> MVTVTDPLTARLEAAIKAWSDFFSDAEHERLDPAIFADQSQTLFANHPLAPVPLADLLLRPTPSNRECVDQRTLQYLQVLQKQGRITTAAVLRALYKYSTAHTRAQTPDGKPKHGAGDSSTNDADVGGSSKADLTSRMVRWRNSYMVEEDVLWRLARAVNHGTGIKTSHDVTEVAKVLARWTALFAEVSAAISRDAFNSMNGLQVKDESEDARNAFVLFYFAFCENQIVNETLSQPVCKDICRKLLDSLDAFLPTLMHLTADITGRLEHFRSEVLARYAPQEKKSMDMPSFMNDLSMSLESFQVPELPVVNTRAGLYIYLGAALVGRPMIDDEALFSYLHNRYQGDLQAMAVHLILASFDLLANAVFRNEGAKTGHLLKSFLINKVPLILVQLVAYAATTMYPFNAEMCITEALNQVDINMFPTLSGMFDMPNNNSFNDSVRQDFCFACQLHGLLSQAAIETLLGDITYQSLPPEGRYVKEQLVQACLQEPDRTLKLIGELDNMNGNVGAAAQAIVEICRDLASKPLSLDVLLLFDKPHKILHPLCELLDNWAGYEEDHGEYQPVYEEFGSVLLLLLAFVYRYNLSTADLGIRSSGSFVAKLLNGVDRCQPLEQLSEQEKSHLGGWIHGLFDTEAGGLGDELMSSCPPQDFYLLAPTLFHQIVNALSAGYLTDEMLKGGLEYLVDVLLLPALVPALLYLSNLLWADNQPIQNAVIKILQPILKPTSISNEASTMLSSVLNIVAKPLEHALKSYQRQDPECQKIEPLLLAIADNLAVSRRTGGADHTELESWCSAQITNPATGALIHGGLAAAVRTTIQQLVQWAQNPTLNSMNGMPAPYTHRQTLAAQQILGPHRLLGIILDELKSSPEPGIAYDVVTTMICAPDVRNSTISSPSTQSNNSSDHNDQAQNHQSQDAKHKHPHRLTLRDALRLEAHDFRAHLRADPVLAETVVRLYRRVEAQLTPLALPLPPAAAAAPAVGVNVGVDAATAAAAAAAAAMMPDALGLGVVGGVELGGMEGAIAAAVAAANGSGTGGAGGDGTQGGAGDAGMGLDGQQQGQGGSSAGDMGLGGGTADDIFSGLSGPDDFGADFGSWSMDLS;> MEARAHGALPNNYDRERFINGVGGDDKALKRKLEEPLSDITKELDTVIAQSDVAVADPKGQLCPDADVPDEMEHITDGILPLNLLLIRLAEFSHSKLEELVTMLASKPVPQHAVNGNGSHSTLVEDASPESQEKKRLLLNTIQDLHSRWVKALVITEWARNAEKVGKLIDIRTHLFKKLELYPQVLNDFINLKRDMAWAKVPSPDLKTALHILTHGEVTWMPDFNFLDPPPLTTEETLRWINDMNLALHARLQLEEHDKLPPPFKNYTIDSGRVTFRVRGEFEVDLSISEEDFSEQFWFINFRFDFSPAPAELTPAVRYWMTEKVNNILKTEGLGGCYKYLHEFTLTQKIAELHRQAIALNKGRWANSLRVEKLNRNLGIHYWANRLHSQNLKSWIIIGVHSGEDPQGLEEPKPSYLMVQWFREGVEQFIDIPFSQEKLSIEEILEFVTAKHVGYLLFSLFRKFDGKPRFTQGKKARLELNVWTQKPEDYYLSMQLLDDEDLKIQVNPWMGDFITTPSTGPWNRTLNSLGNPAEEGSKELENFRYIYIISVLKAQGKSHGWSVVRSPISQDELRSIVHSESASSRETFQAAWTRFVDWDPQWYAMRSMSLAGDQWWLVEVTSQRQSISGNRLVFFTKMAPCFSEERLTDGFFNGLRDHSRRLIAEITNLRELYPGITPSQLRKLIDPTRQPPVLPVKASKILGDFGGADAQSIAWLKDPVWLIYRGSACDTRVSDSPQQKRTQPVLDVFEAYLDVTDRRRFQTLNPRLDRDILYNPYTGRFMFRLRAKMGVPVVPLLGIRVRQLQRLLDFLEGLRRVGDDAVPERVTLREIVFSYGATRKRDSTNQPKVRPWRVRLDLTKEEGVGVVLEKGNPHLRVINRLEDLVNSQKFYSLATYLTLSLPLFRAFQQLENAWQTAQENGRGSCFILHLSLDKHTIRFVLPGHQRQISLLIQPHEKEGKLVWEVGRPRHDPELLNENCEFNRVLKERVWTISGSGFKGLVTGAAAEPDEGIERLLVLISDAVLHLSTSQPATAPPQPPQAQPSQQVQQVQQQQVVSQLQPQAQQPRSAMPHASVGQQQPHGAPAPMARFPPQQQQIFQQQRPPQPQPNMHGGQISQPNMHGGPKPQLQGQHGQPGQMVAAPQQQGQRPGTGTAAGMGRSNAPLVVLD;> MAANIPQFPNGQMAMLQQQQQQAQQQAIAANQQYMNVFILNNLRGSGTNLPGTWQAQIPPQQLLSERFQKTHILYTNIMLASNGGDPQRCAVAALNLEKQIFQNAQDKASYDQAMAKKISEVMKRRESNGPALQNQVITDAQRQAQIQQQIQLAQAQQRQQQQLMLNRMAAQGLTQPPQPAFQPMQNPGQVPVIPQQMGINVAVPGMLPNAPSQPQLAMQMGQPRPGAIPVDLNQLSNQDRMRIHEEVMRRVNSTTENSKMQIRQLMQQRLTPAQISEANASGKDLVYLYFQNQVVQVFRATMLQAQEKAQQVAQVQQALLMQQRQGIQGAGMPGVPPQGQVNPALMNALGQQPAISDAPMLGPNLTNEPQMGLLAQQPGQMIVPTNPAAVPGRPVTAGPQLGAIPPQPTPGNPQAPNQTPRPGQLQQPFGMPQVNNPAAAAAAAAAAAAVQQPPQAQPGMRPPGPRTMPGQPGAITTVAGPQPTSQSPAMNTLNAPMRQPPVAMTQATTQPVNPANAPMAGATLNAQFNHQNNARPLSMQGNMNNQAMAGMGAAANMNANNNPMKEFMARLQEQQRATAAAGFQGPKPGQVIGMPGQFPGGPMNALNQPGMFNQNSKPNAMVPPTAQAAALQQQQQQANAADMANIYKIIQTPQGQNMMNNMDIHQMILQEINKHLGGRLPPNITKWAHLRQFLAAQPNALPSEIVQRIMSYQILQFKNFWKRASQPNAVGGIPQPVSNVPVSQFAGMNQPVAPPPGVQVPQSISQVSPQDIEGLRKNPKFANLTDDQLAEWIRKVKQQSFIKKAWEIHNNQSNAAQNQATNSSLIGQQKPGMTVPPTPTTAQPTSSVVQTAQSRPQGPQPTPTPQGPQGVQPQAAQPKPTPSPAANVTTAPPATTGMSAASVQAANIRPSMPQQQQQPAPQPQAPQPPPPQQQQQQQQQQQQQQQQQQQQVPQPPQNSRQAPMDPSPAMATKSLKRPSPDDSAEDTPAQQNITPMQRAPSQAAQVAPNAPNAASGEPPKLSPELQKLRNLASEAQLEVSKEHLQPILMTPADQQETREKIAQVKLKMNQIRSMGLLPKWYYLTNDDNRARQFFRGRFKVVKQFTDGEAMTQLRDTFTITKEELNQYDNLLGSMLRDMMMSRVNQQQAAMMNQQQQTQQQTTQPTPATLANQQAAALRQAQQRVAPPPPKPVQQPPAQQQQPHQPAQPAQQQFQPGVQPTPAPAPEYFGDQRLTAANLVLPPRKKPKVSGNQTSPSANQQLAAGSPQVQALSPVATRKPEPQVKPQAQIPQQQQQQQQQQQQQQQQQQPQAPPAPQFKCPEPGCTSLVAFPSEEALNAHRQEEHLKPAENPLAFMQEQMASVLALDAQGRAKASPKPSGQDVSTPVPTAPPMSASLSKQGQTPRLQAATPMSRNLSMQRQGSASGGKPGENMPTPGKSAGGKGKEGATPQQMEDVWPQGTIDPANLFANLGGTLDAGTATISGSIITDFAAYRSSTPKDTPESSSSSKDSGVSEPNSDINENANLEIDLFWSNIDDGLLMDINNISMDGAAGSMGGSSGNAGGLVDISQFVEDPWGVDSANFSLDDFGRELDKGFGFLDGTLGEGQQESGQGQGQGQPEVMVIE;> MALLMEGGDPMSVDGSSTMPAHMRVMPDMGITGAPMTLDDVDLFGDAVMNNALDALPPAPGHPPPSRALQRRIAELRARGCCQGIAWSRQGTIASISADGMSIELRFLRTNPENGDWELTDAALSLSVALVPASSPSATSSSGSGTSNTTVISAGAPFVHLAWAPSVHTSSFELAAIDAPGRITIFLFTQNINKPYLSRKWDTDPVDDLHAVVGCYWLPLPFNVSYVANWVQTDYRYEPILSPAWGPIHPNHTKSALVCVTTNGLLKMLFPQNNNRIEETSIELESVTASDDLITHAAIGADRNTLLIALAMGSKQLRVVRVGIQWWLPQVDKQQMPPSVPLRPSLRESRVAVTTLLDPEQQQSDGDAPIAQLTHLEILPSPLGETPQTVLPPVILAVRSYLPQEGSLYAAHQEPFTVIDRWELFTDQPKAFHPAFEQLGAKNSASSQPSAMQTLRKLDPVVIPGKVVVTVNTLQFGRVVCFGFSDGTLQYRDRFTMNEVYTEQATTNITSPLQVGFQWETEGPCLQMAFAPTNCSFVQVSEDGSVKWVKLRYPVDDPNMTLQGPKLKAVAASLAVASVGANIAGPNIHNHCDDVMAIARPLAKKFKDFPTAWVREFVTMFKITVDYSEEAHHDQLMRNSLLQFCLSILNHFGFNGDFQPRTFSGKFANLALAVRNIVVLITIASNAPNTIKEKLSPLDEPEVVDALASCAKWGFDLLAWLTDRLLALSTDQTIKAMLADQKRFPDLARYLHSKNDVSLHLLLCSSTRGLLSAVCRRLQVVESLAHRATVYYESRYAVDPAAAAQKTLPPLYHAYVKMQRVVTASLVKASDFDKLLTALSRDIQTAYIQTFSGVATQIRQHASGSGGQPLTEQQQQQCNEQFIKKAQSHVELDMLLGQNPPPGFREVLACFFGNIFPAFRATVDPRSVFFADWSLLEEIVAEDERTLKRRREGGGRYVDVFKRVELCGRGQVLPRGRIVASVKTERAEAVPMVPSQSQSSHQAASQAQGQQSQQQQGATPAPNATPSVPISQLNPPTGPTQPPNSSGNTA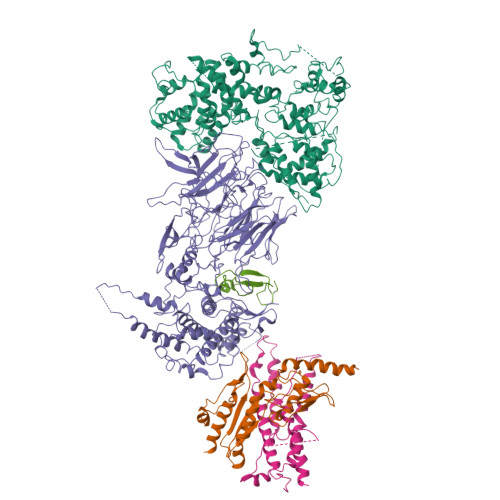NANPNTGTNANTLGGSVPGLQGFVPVTANLAVNASQWRRCVRCAAVMEDVWGQRPGFTFVLTQQRRCACGGGWGLVPRGD>AAEASKKPRQKRTATKAYNVTQAFGRRGPEQTQGNFGDQELIRQGTDYKHWPQIAQFAPSASAFFGMSRIGMEVTPSGTWLTYTGAIKLDDKDPNFKDQVILL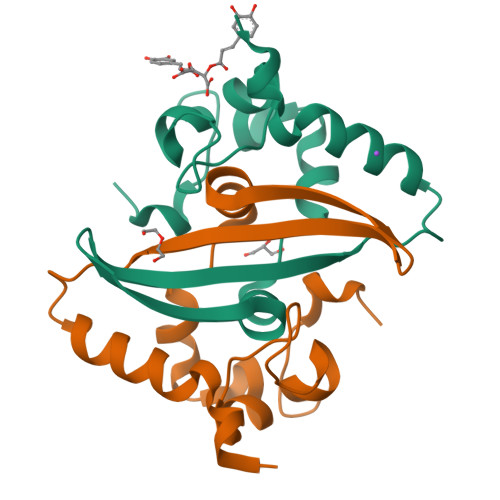NKHIDAYKTFP[6x]> AKKYAVVLKTLTDPFWQSMKAGIEAEAKELGVTVDIFAAASEGDAEAQLALFESLSNKNYKGIAFAPLTADNLVEPVASAWKKGTYLVNLDDKIDMKALKAAGGNVEAFVTTDNVAVGAQGAGYIIEKLGAEGGEVAIIEGEAGNAAGEARTKGATDAFDKASNIKLVASQPADWDRAKAKQVATDILAKHPNIKAIYCANDTM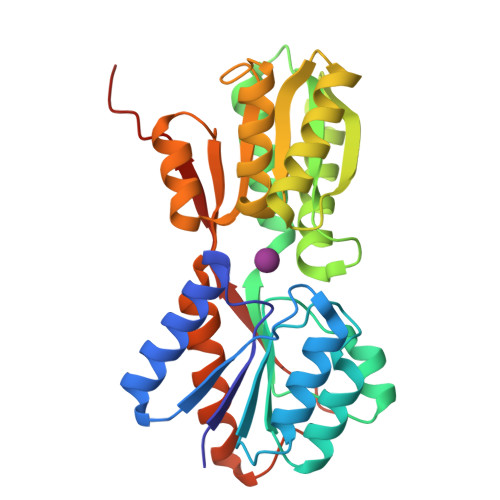ALGVAQAVADAGKTGKVLVVGTDGIPEAQQAVKAGKMTATVAQNPAAIGATGLKLMVDAQKKGKVIPLDKKPQYVLVASKLVTKLEHHHHHH> MKSNDMNITVELTFFEPYRLVEWFDWDARKKSHSAMRGQAFAQWTWKGKGRTAGKSFITGTLVRSAVIKAVEELLSLNNGKWEGVPCCNGSFQTDESKGKKPSFLRKRHTLQWQANNKNICDKEEACPFCILLGRFDNAGKVHERNKDYDIHFSNFDLDHKQEKNDLRLVDIASGRILNRVDFDTGKAKDYFRTWEADYETYGTYTGRITLRNEHAKKLLLASLGFVDKLCGALCRIEVIKKSESPLPSDTKEQSYTKDDTVEVLSEDHNDELRKQAEVIVEAFKQNDKLEKIRILADAIRTLRLHGEGVIEKDELPDGKEERDKGHHLWDIKVQGTALRTKLKELWQSNKDIGWRKFTEMLGSNLYLIYKKETGGVSTRFRILGDTEYYSKAHDSEGSDLFIPVTPPEGIETKEWIIVGRLKAATPFYFGVQQPSDSIPGKEKKSEDSLVINEHTSFNILLDKENRYRIPRSALRGALRRDLRTAFGSGCNVSLGGQILCNCKVCIEMRRITLKDSVSDFSEPPEIRYRIAKNPGTATVEDGSLFDIEVGPEGLTFPFVLRYRGHKFPEQLSSVIRYWEENDGKNGMAWLGGLDSTGKGRFALKDIKIFEWDLNQKINEYIKERGMRGKEKELLEMGESSLPDGLIPYKFFEERECLFPYKENLKPQWSEVQYTIEVGSPLLTADTISALTEPGNRDAIAYKKRVYNDGNNAIEPEPRFAVKSETHRGIFRTAVGRRTGDLGKEDHEDCTCDMCIIFGNEHESSKIRFEDLELINGNEFEKLEKHIDHVAIDRFTGGALDKAKFDTYPLAGSPKKPLKLKGRFWIKKGFSGDHKLLITTALSDIRDGLYPLGSKGGVGYGWVAGISIDDNVPDDFKEMINKTEMPLPEEVEESNNGPINNDYVHPGHQSPKQDHKNKNIYYPHYFLDSGSKVYREKDIITHEEFTEELLSGKINCKLETLTPLIIPDTSDENGLKLQGNKPGHKNYKFFNINGELMIPGSELRGMLRTHFEALTKSCFAIFGEDSTLSWRMNADEKDYKIDSNSIRKMESQRNPKYRIPDELQKELRNSGNGLFNRLYTSERRFWSDVSNKFENSIDYKREILRCAGRPKNYKGGIIRQRKDSLMAEELKVHRLPLYDNFDIPDSAYKANDHCRKSATCSTSRGCRERFT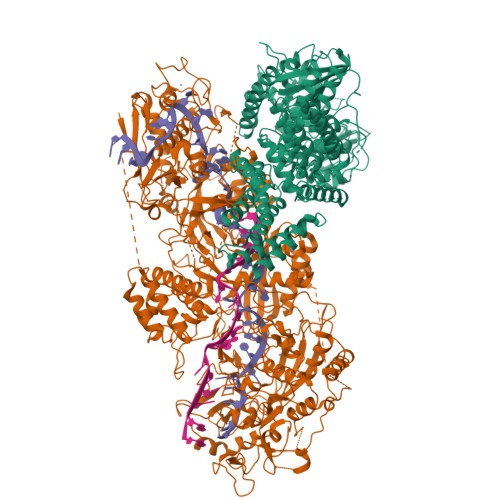CGIKVRDKNRVFLNAANNNRQYLNNIKKSNHDLYLQYLKGEKKIRFNSKVITGSERSPIDVIAELNERGRQTGFIKLSGLNNSNKSQGNTGTTFNSGWDRFELNILLDDLETRPSKSDYPRPRLLFTKDQYEYNITKRCERVFEIDKGNKTGYPVDDQIKKNYEDILDSYDGIKDQEVAERFDTFTRGSKLKVGDLVYFHIDGDNKIDSLIPVRISRKCASKTLGGKLDKALHPCTGLSDGLCPGCHLFGTTDYKGRVKFGFAKYENGPEWLITRGNNPERSLTLGVLESPRPAFSIPDDESEIPGRKFYLHHNGWRIIRQKQLEIRETVQPERNVTTEVMDKGNVFSFDVRFENLREWELGLLLQSLDPGKNIAHKLGKGKPYGFGSVKIKIDSLHTFKINSNNDKIKRVPQSDIREYINKGYQKLIEWSGNNSIQKGNVLPQWHVIPHIDKLYKLLWVPFLNDSKLEPDVRYPVLNEESKGYIEGSDYTYKKLGDKDNLPYKTRVKGLTTPWSPWNPFQVIAEHEEQEVNVTGSRPSVTDKIERDGKMV;> MNNTEENIDRIQEPTREDIDRKEAERLLDEAFNPRTKPVDRKKIINSALKILIGLYKEKKDDLTSASFISIARAYYLVSITILPKGTTIPEKKKEALRKGIEFIDRAINKFNGSILDSQRAFRIKSVLSIEFNRIDREKCDNIKLKNLLNEAVDKGCTDFDTYEWDIQIAIRLCELGVDMEGHFDNLIKSNKANDLQKAKAYYFIKKDDHKAKEHMDKCTASLKYTPCSHRLWDETVGFIERLKGDSSTLWRDFAIKTYRSCRVQEKETGTLRLRWYWSRHRVLYDMAFLAVKEQADDEEPDVNVKQAKIKKLAEISDSLKSRFSLRLSDMEKMPKSDDESNHEFKKFLDKCVTAYQDGYVINRSEDKEGQGENKSTTSKQPEPRPQAKLLELTQVPEGWVVVHFYLNKLEGMGNAIVFDKCANSWQYKEFQYKELFEVFLTWQANYNLYKENAAEHLVTLCKKIGETMPFLFCDNFIPNGKDVLFVPHDFLHRLPLHGSIENKTNGKLFLENHSCCYLPAWSFASEKEASTSDEYVLLKNFDQGHFETLQNNQIWGTQSVKDGASSDDLENIRNNPRLLTILCHGEANMSNPFRSMLKLANGGITYLEILNSVKGLKGSQVILGACETDLVPPLSDVMDEHYSVATALLLIGAAGVVGTMWKVRSNKTKSLIEWKLENIEYKLNEWQKETGGAAYKDHPPTFYRSIAFRSIGFPL> GPMSEAADVERVYAAMEEAAGLLGVACARDKIYPLLSTFQDTLVEGGSVVWFSMASGRHSTELDFSISVPTSHGDPYATVVEKGLFPATGHPVDDLLADTQKHLPVSMFAIDGEVTGGFKKTYAFFPTDNMPGVAELSAIPSMPPAVAENAELFARYGLDKVQMTSMDYKKRQVNLYFSELSAQTLEAESVLALVRELGLHVPNELGLKFCKRSFSVYPTLNWETGKIDRLCFAVISNDPTLVPSSDEGDIEKFHNYATKAPYAYVGEKRT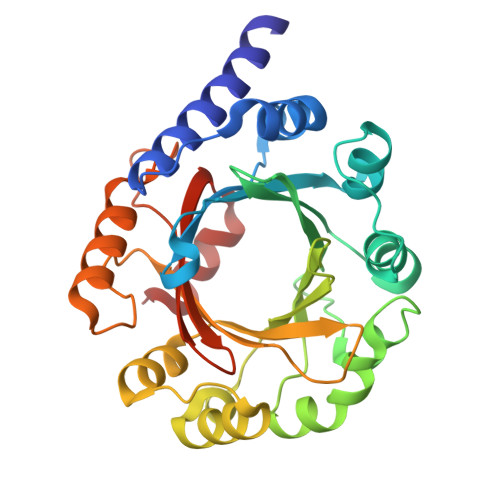LVYGLTLSPKEEYYKLGAYYHITDVQRGLLKAFDSLED>[2x]GMADAPIDIFQSILSRKSIRAFTDQPVTQETIREILKLAARAPSGTNLQPWQVIVLTGKILQKVGQELSQLVLSGIKGEREYH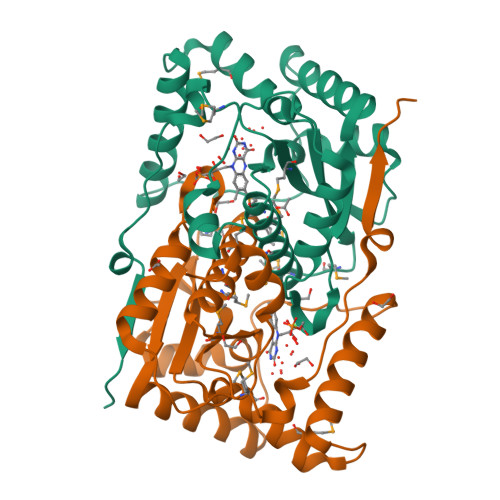YYPRQWREPYLSRRRKVGLDLYKSLGIQKGDQEKMLHQKAKNFLFYGAPVGLLFTIDHDMEMGSWLDLGMFMQTIMLAARGFGLDTCAQAAFADYHKQIRSLLSVPSDRHIICGMALGYRDMNAPENNFETEREPIDNFVHFIKSYP(3~{a}~{R})-2,3,3~{a},4-tetrahydropyrrolo[1,2-a]indol-1-one | C11 H11 N O | 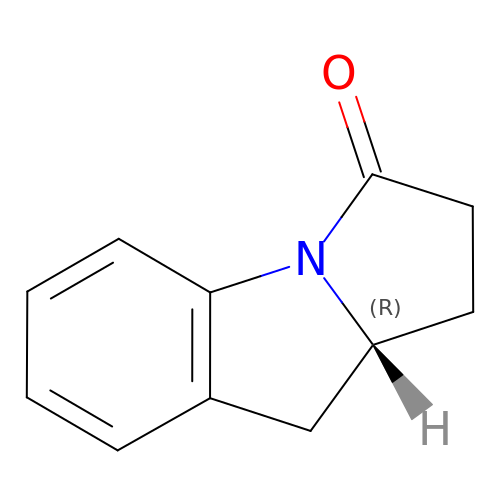QPPMCKRHXDXQPA-SECBINFHSA-N> PF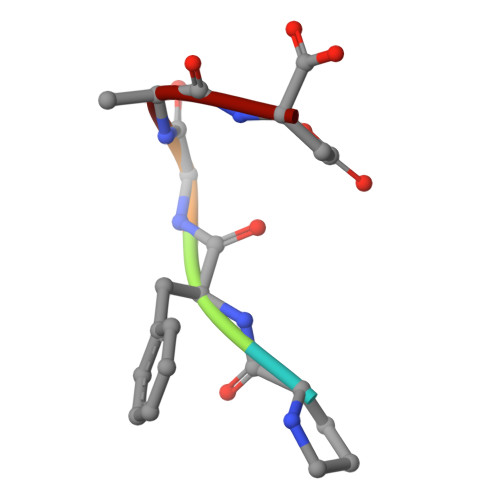GAD>MGSSHHHHHHSSENLYFQGHMKRLEVSNQAKLPTQFGEFYIQCFREKGSNGSKDHLVVFTPNFSQNPLVRLHSECLTGDALGSQKCDCGGALQMALERISKEGGLVIYLRQEGRGIGLFNKVNAYALQDKGYDTIQANEMIGFKDDERDY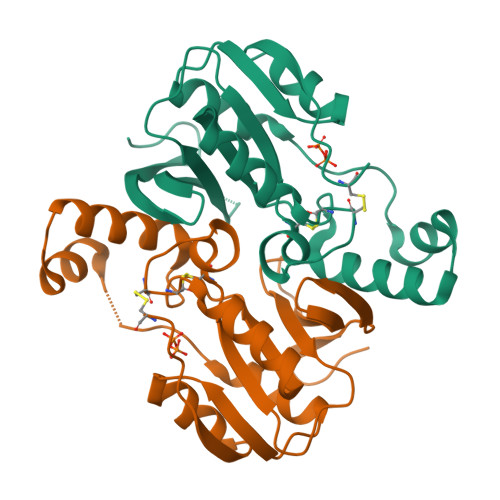SVAGEILEYYRIKKMRLLTNNPKKIAALEKYAEVTRESLIVCANEHNQGYLEVKKLKMGHLL[2x]>MHHHHHHSS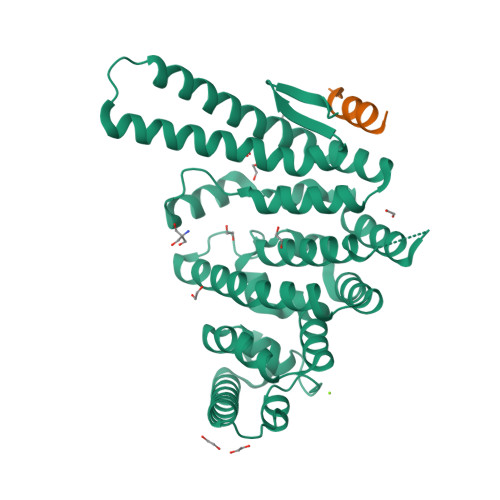GSSSTGSSAAAVASKQRRRSSYAFNNGNGATNLNKSGGKKFILELIETVYEEILDLEANLRNGQQTDSTAMWEALHIDDSSYDVNPFISMLSFDKGIKIMPRIFNFLDKQQKLKILQKIFNELSHLQIIILSSYKTTPKPTLTQLKKVDLFQMIILKIIVSFLSNNSNFIEIMGLLLQLIRNNNVSFLTTSKIGLNLITILISRAALIKQDSSRSNILSSPEISTWNEIYDKLFTSLESKIQLIFPPREYNDHIMRLQNDKFMDEAYIWAFLASLAASGKLNHQRIIIDEVRDEIFATINEAETLQKKEKELSVLPQRSQELDTELKSIIYNKEKLYQDLNLFLNVMGLVYRDGEISELK[2x];>TSGSNELLSILHRK[2x]> MGGSHHHHHHMASSVPIPGIKDISKLKFFYGFKYLWNPTVYNKIFDKLDLTKTYKHPEELKVLDLYPGVGIQSAIFYNKYCPRQYSLLEKRSSLYKFLNAKFEGSPLQILKRDPYDWSTYSNLIDEERIFVPEVQSSDHINDKFLTVANVTGEGSEGLIMQWLSCIGNKNWLYRFGKVKMLLWMPSTTARKLLARPGMHSRSKCSVVREAFTDTKLIAISDANELKGFDSQCIEEWDPILFSAAEIWPTKGKPIALVEMDPIDFDFDVDNWDYVTRHLMILKRTPLNTVMDSLGHGGQQYFNSRITDKDLLKKCPIDLTNDEFIYLTKLFMEWPFKPDILMDFVDMY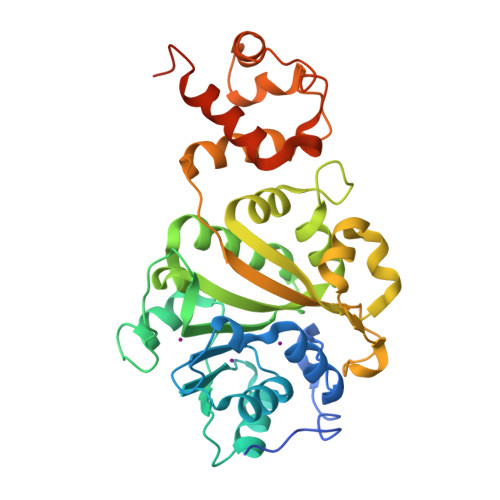QTEHSG>XGEIAQAXKEIA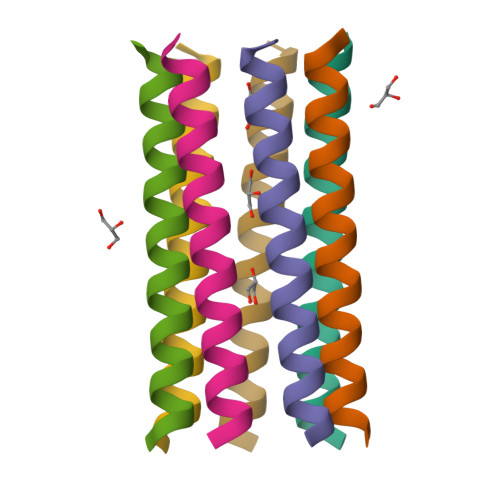KAXKEIAWAXKEIAQAXKGX[7x]> MDWPHAGRPAHEL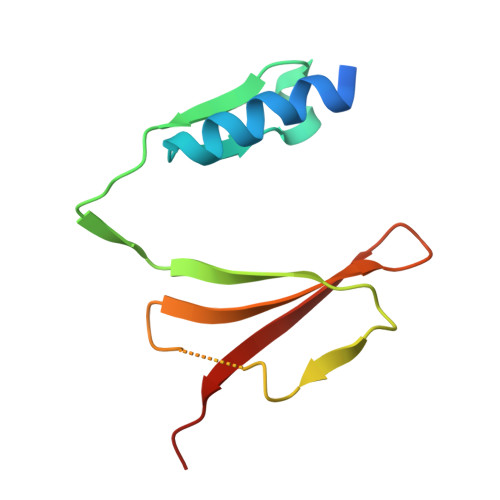RYSIYRDLWERGFFLSAAGKFGGDFLVYPGDPLRFHAHYIAQCWAPEDTIPLQDLVAAGRLGTSVRKTLLLCSPQPDGKVVYTSLQWASLQ>MARGVNKVILVGNVGGDPETRYMPNGNAVTNITLATSESWKDKQTGQQQERTEWHRVVFFGRLAEIAGEYLRKGSQVYVEGSLRTRKWQGQDGQDRYTTEIVVDINGNMQLLGGRHHHHHH[4x]

Single-stranded DNA (ssDNA)-binding protein (SSB) plays a crucial role in DNA replication, repair, and recombination as well as replication fork restarts. SSB binds to ssDNA with a high affinity regardless of the sequence and prevents premature annealing, chemical attacks, and unwanted nuclease digestion. Bacterial SSBs typically recognize ssDNA via a highly conserved oligonucleotide/oligosaccharide-binding (OB) fold formed from a five-stranded β-barrel capped by an α-helix. In this study, the effect of the flavonols myricetin, quercetin, kaempferol, and galangin on the inhibition of Pseudomonas aeruginosa SSB (PaSSB) was investigated.

The complexed crystal structure of PaSSB with quercetin was determined at a 2.3 Å resolution. Four monomers of PaSSB were found in the asymmetric unit. A quercetin molecule could be found in a cavity created at the interface of PaSSB monomers A and C. However, unlike the complexed structure of PaSSB with myricetin, which contained two myricetin molecules per tetramer, only one quercetin molecule was found in the structure of the PaSSB tetramer. Having a similar binding site to myricetin, but with a different binding pose, the quercetin molecule was sandwiched between PaSSB monomers A and C. The binding of quercetin did not influence the overall structure of PaSSB. Residues Ile105 (monomers A and C), Asn106 (monomer A), Gly107 (monomer A), and Asn108 (monomer C) within contact distance (<4 Å) were involved in quercetin binding. Gly107 and Asn108 formed hydrogen bonds with quercetin. In addition, compared with myricetin, the aromatic ring of quercetin shifted by a distance of 4.9 Å and an angle of 31° for hydrogen bonding to the side chain of Asn108 in PaSSB. Based on our crystal structure, we found that in the absence of one OH group, compared with myricetin, quercetin could not interact with Lys7 and Glu80. Thus, quercetin did not inhibit the ssDNA binding activity of PaSSB.>MVKQIESKTAFQEALDAAGDKLVVVDFSATWCGPCKMIKPFFHSLSEKYSNVIFLEVDVDDCQDVASESEVKS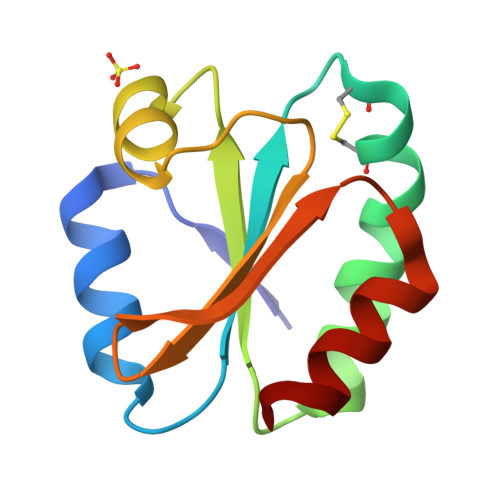MPTFQFFKKGQKVGEFSGANKEKLEATINELV[2x]> MPSQNALYLDLLKKVLTNTIYSDRPHPNAWQDNTDYRQAARAKGTDWPTVAHTMIGLERLDNLQHCVEAVLADGVPGDFAETGVWRGGACIFMRAVLQAFGDTGRTVWVVDSFQGMPESSAQDHQADQAMAL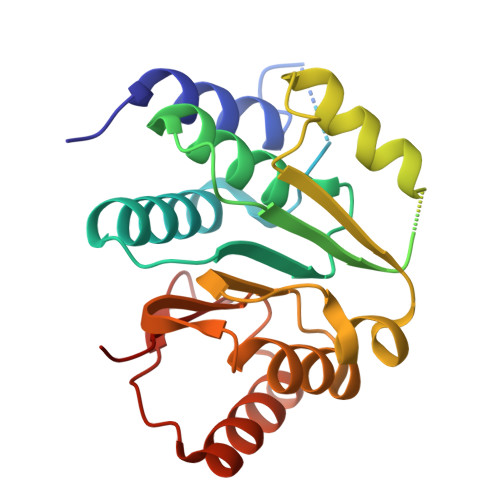HEYNDVLGVSLETVRQNFARYGLLDEQVRFLPGWFRDTLPTAPIQELAVLRLDGDLYESTMDSLRNLYPKLSPGGFVIIDDYFLPSCQDAVKGFRAELGITEPIHDIDGQGAYWRRSW>[2x]MRTFESVADLAAAAGEKVGQSDWVTITQEEVNLFADATGDHQWIHVDPERAAAGPFGTTIAHGFMTLALLPRLQHQMYTVKGVKLAINYGLNKVRFPAPVPVGSRVRATS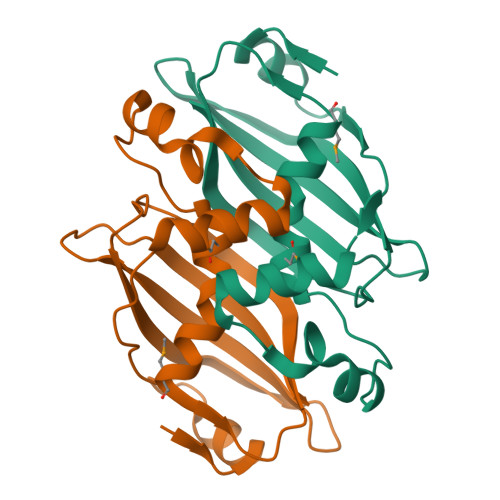SLVGVEDLGNGTVQATVSTTVEVEGSAKPACVAESIVRYVA> ETGAAADWDVYCSQDESIPAKFISRLVTSKDQALEKTEINCSNGLVPITQEFGINMMLIQYTR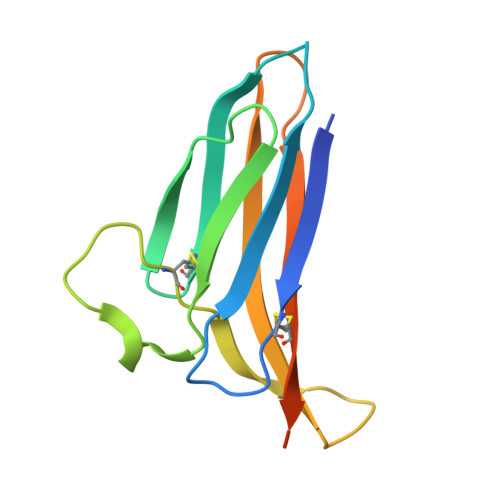NELLDSPGMCVFWGPYSVPKNDTVVLYTVTARLKWSEGPPTNLSIQCYMPKSPVAPKLEHHHHHH>[2x]AKPCTVSTTNATVDLGDLYSFSLMSAGAASAWHDVALELTNCPVGTSRVTASFSGAADSTGYYKNQGTAQNIQLELQDDSGNTLNTGATKTVQVDDSSQSAHFPLQV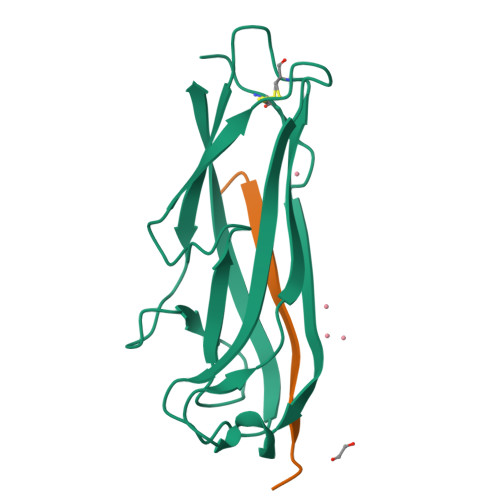RALTVNGGATQGTIEAVIEITYTYS;>ADSRIRIRGYVRNNG[2x]3,4-DIMETHYLANILINE | C8 H11 N | 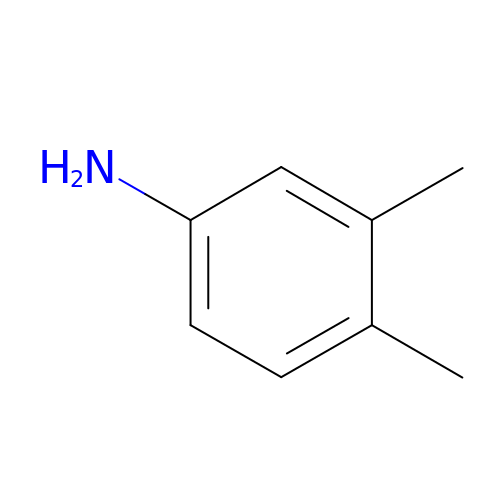DOLQYFPDPKPQSS-UHFFFAOYSA-N2-[4-bromo-3-(3-chloro-5-cyanophenoxy)-2-fluorophenyl]-N-(2-chloro-4-sulfamoylphenyl)acetamide 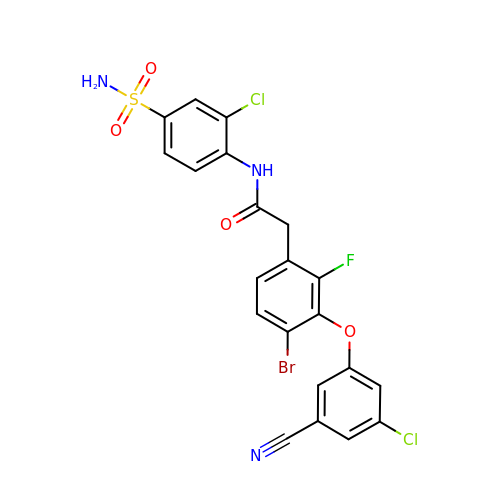| C21 H13 Br Cl2 F N3 O4 S | SBUUICLVCQQMFP-UHFFFAOYSA-N>[4x]MMALDDTVTIKPIRAEHVESFHRALDAVSRERKYLSFLEAPPLEAVRAFVLDMIENDHPQFVAIADGDVIGWCDIRRQDRATRAHCGTLGMGILPAYRNKGLGARLMRRTLDAAHEFGLHR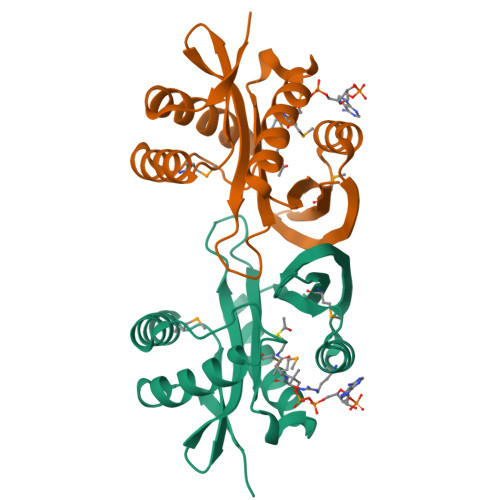IELSVHADNARAIALYEKIGFAHEGRARDAVSIDGHYIDSLNMAIIFGN>[3x]MFESMKPHLAELRQRLAISVL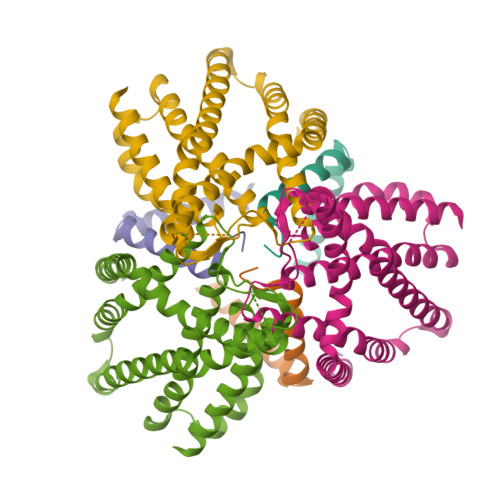AVFVGFIIAFTFHNAILGWITKPLNNALIQVGKIVEKREMGTWKISGNEHNATLAPSKSPALLSDHAQSAEKLHRTLAEASQATQNPKLQKLLSQAASAAEELARNSRILRKALVKEENLTRQAVNQNLREKSFNGMITTHQVGGAFFVALKVSFFAGILMAMPVILWQLWLFIAPGLYDNEKKMVLPFVVGGSVMFLIGVLFAYYVVTPFGFQFLITFGSFLYTPLINIEDYVGFFTKILIGFGIAFELPVVAYFLALLGLITDKTLKDYFKYAIVIIFLLAAFLTPPDVLTQLLMAAPLILLYGLSILIVHYVNPYKPEEKEDDEEEEEDEFEKAEREFEALEKGSESHESGSENLYFQ;>[3x]MFGMGFSEILVIALVAILFLGPDKLPEAMVQIAKFFNSVRKTINEAKSTFEEELHLKELKEEALSYRQSLSEVGSDISGFKNAISNHTDELQEAIEIARSGMPTDRLNESVDDLLEEDEPTGETSQRPGVTEYKEMARKALEEAENSAEAQTAETPSVEDKGPESSPKESSRPAGFKHLDNEANAWSHPQFEK Here, activity screening of a metagenomic library created from rumen fluid led us to the isolation of a novel β-glycosidase, GlyA1, which was assigned to the GH3 family. Activity was confirmed for 18 substrates that revealed that GlyA1 is a GH3 member with clear β-glucosidase and β-xylosidase activities, but also possessing β-galactosidase, β-fucosidase, α-arabinofuranosidase, and α-arabinopyranosidase activities at low level in this order. Structural analysis illustrates the permuted domain composition of GlyA1 that is composed of an N-terminal (α/β)6-sandwich domain, followed by the FnIII domain, and the (α/β)8 barrel domain. The active site of GlyA1 is located at the molecular surface, at the interface between the (α/β)8 barrel domain, which provides the nucleophile Asp-709 and the (α/β)6-sandwich domain, contributing to the Glu-143 acid/base catalyst.

The low numbers of crystals impeded analysis of the intact protein by mass spectrometry, but SDS-PAGE analysis of protein solution samples revealed the presence of two bands after incubation at room temperature or treatment with proteases. Therefore, the sample was incubated with subtilisin previously to the crystallization step, which accelerated formation of many good quality crystals, under similar conditions and with the same space group. These crystals were cryoprotected into 20% glycerol, and this molecule was found bound at the active site. Interestingly, the last loop is markedly flexible as it is deduced from the fact that it could only be fully traced in the ligand-free crystal, containing only glycerol in the active site, and in the galactose-soaked crystal of the truncated form. Xylose and glucose are bound in an identical position, and the glycerol molecules observed in the ligand-free crystals are mimicking the positions occupied by C2, C3, C4, and C5 from both sugars. Furthermore, the traced loops showed significant conformational changes in the different crystals at Trp-111, coupled to a change in Phe-147 from the adjacent 139–152 loop, reinforcing its intrinsic mobility.

> MNIEKVILDWNEYIEAARSVVSEGCVLLENNGTLPLEKGAVVSIFGRIQTHYYKSGTGSGGMVNVTHVVGVPEGLKLSEHVTVNEELENIYKEWEEENPFDEGLGWGTEPWSQPEMELTDEIVSNASAKSDVAIVIIGRTAGEDKDFSDVAGAYKLSETEEDMLRRVRKHFDKMVVLLNVGSLMDLNVISEINPDALMVIWQGGMIGGLGTADVLTGKVNPSGKLTDTIAYEINDYPSTENFGDPVRDYYAEDIYVGYRYFETFEKSKVRYPFGYGISYTEFEHTVGEFTADINSRTFTASCTVKNTGSVAGKDVAQFYVSAPQGKLGKPEKVLVAFKKTGILNPGKEEKITVTVPFDRFASFDDTGVTGAESCFVLEAGEYTVYEGKNVRESYKEGSFTLEENIVTEKLSKALAPMESFKRMKASENSDGTLSVKYEDVPVSDVDEKKRRLDNMPVEIPQDFTARYSLKDVLSGSVDMEKFIARLSDDDLACIVRGEGMGSSLVTAGTAAAFGGVSEYLRKMDIPAVCCDDGPSGMRLDSGATAFSMPNGTMLASTFNPDVIERMYGFTSLEMIYNKVECLLGPGMNIHRNPLNGRNFEYFSEDPYLNGTIASAMLKGLHKYGSDGVAKHFCCNNQELGRQACDSVVSQRALREIYLKGFEIAVKEGGCKAFMTTYAQVNGMWTAGNYDLNTRILRDEWGFKGIVMTDWWAQVNDRGGEPTKNNTAAMVRAQNDLYMVTANAAMNSANDNTLSQLSEGKLNRAELQRCAMNICEYAMNTMAMKRLCRNDIKVEIAGRVIEEDAFDIENAEYLVLKGNITVSLKNKESKAGTNYYIPLDIQDLGMYDISVTASSMLGEVAQLPCTLYYTGVPFLTYTFNGSGGKDVTITKSMDFHNRMAVIRLNVAKNGLNLDRIEFKKQQ>[8x]SNAMRNRIEQALQQMPASFAPYLRELVLAKDFDATFSAEQYQQLLTLSGLEDADLRVALLPIAAAYSYAPISEFYVGAIVRGISGRLYLGANMEFTGAQLGQTVHAEQCAISHAWMKGEKGVADITINFSPCGHCRQFMNELTTASSLKIQLPKRAAKTLQEYLPESFGPADLGIDS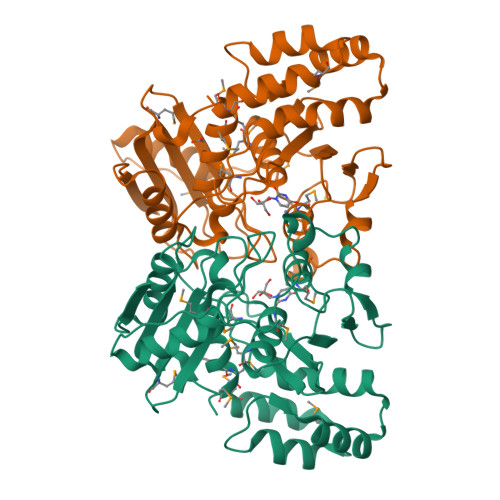GLMSPVNHGKTSDDDEELIQQALRAMNISHSPYTQNFSGVALKMRSGAIYLGAYAENAAFNPSLPPLQVALAQAMMMGESFEDIEAAALVESATGKISHLADTQATLEVINPDIPLSYLSL>[2x]SMEEEI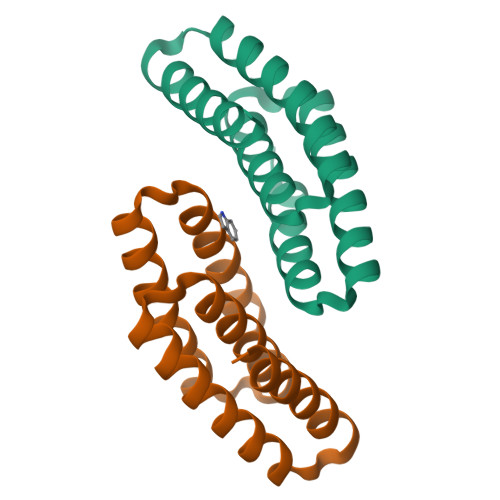EEAYDLVEEAEKTGDTSLLKKAKELLDKVAEEATKSGNPILLIRVIIILIKIVRNSGDPSVAALARELLEKLEEIAEKEGNRFIEAMGEALRTQIERAL>[2x]VGPKTGEENQVLVPNLNPTPENLEVVGDGFKITSSINLVGEEEADENAVNALREFLTANNIEINSENDPNSTTLIIGEVDDDIPELDEALNGTTAENLKEEGYALVSNDGKIAIEGKDGDGTFYGVQTFKQLVKESNIPEVNITDYPTVSARGIVEGFYGTPWTHQDRLDQIKFYGENKLNTYIYAPKDDPYHREKWREPYPESEMQRMQELINASAENKVDFVFGISPGIDIRFDGDAGEEDFNHLITKAESLYDMGVRSFAIYWDDIQDKSAAK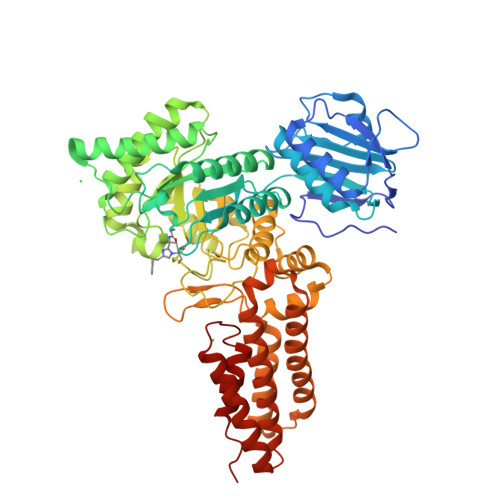HAQVLNRFNEEFVKAKGDVKPLITVPTEYDTGAMVSNGQPRAYTRIFAETVDPSIEVMWTGPGVVTNEIPLSDAQLISGIYDRNMAVWWNYPVTDYFKGKLALGPMHGLDKGLNQYVDFFTVNPMEHAELSKISIHTAADYSWNMDNYDYDKAWNRAIDMLYGDLAEDMKVFANHSTRMDNKTWAKSGREDAPELRAKMDELWNKLSSKEDASALIEELYGEFARMEEACNNLKANLPEVALEECSRQLDELITLAQGDKASLDMIVAQLNEDTEAYESAKEIAQNKLNTALSSFAVISEKVAQSFIQEALSFDLTLI> MDSRLSAAYAIRAARIS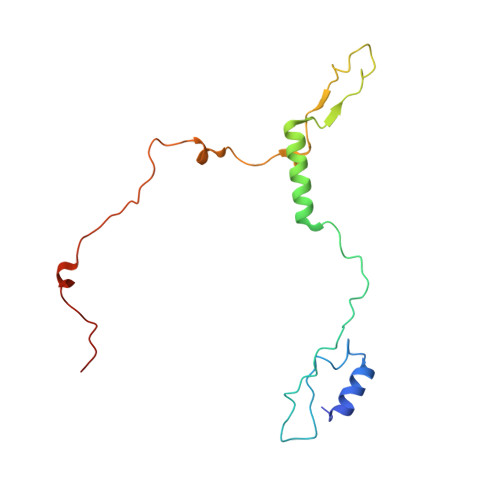MIPGGVDGLVINYAEGGEPAWVQYPLKKQKPLPNNLCYTPTLEDIARKREAVIAKYTKQPLETGTTFTHVLNASHLNEQYTRVKKSALPDKEFPIIETEKYPEPPILWETTIGAPSRLFDRSDGVKYVR> VEFNTDVLDAADKKNIDFTRFSEAGYVLPGQYLLDVIVNGQSISPASLQISFVEPQSSGDKAEKKLPQACLTSDMVRLMGLTAESLDKVVYWHDGQCADFHGLPGVDIRPDTGAGVLRINMPQARLEYSDATWLPPSRWDDGIPGLMLDYNLNGTVSRNYQGGDSHQFSYNGTVGGNLGPWRLRADYQGSQEQSRYNGEKTTNRNFTWSRFYLFRAIPRWRANLTLGENNINSDIFRSWSYTGASLESDDRMLPPRLRGYAPQITGIAETNARVVVSQQGRVLYDSMVPAGPFSIQDLDSSVRGRLDVEVIEQNGRKK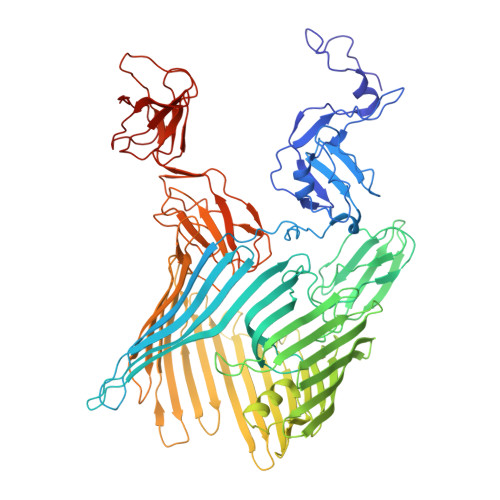TFQVDTASVPYLTRPGQVRYKLVSGRSRGYGHETEGPVFATGEASWGLSNQWSLYGGAVLAGDYNALAAGAGWDLGVPGTLSADITQSVARIEGERTFQGKSWRLSYSKRFDNADADITFAGYRFSERNYMTMEQYLNARYRNDYSSREKEMYTVTLNKNVADWNTSFNLQYSRQTYWDIRKTDYYTVSVNRYFNVFGLQGVAVGLSASRSKYLGRDNDSAYLRISVPLGTGTASYSGSMSNDRYVNMAGYTDTFNDGLDSYSLNAGLNSGGGLTSQRQINAYYSHRSPLANLSANIASLQKGYTSFGVSASGGATITGKDAALHAGGMSGGTRLLVDTDGVGGVPVDGGQVVTNRWGTGVVTDISSYYRNTTSVDLKRLPDDVEATRSVVESALTEGAIGYRKFSVLKGKRLFAILRLADGSQPPFGASVTSEKGRELGMVADEGLAWLSGVTPGETLSVNWDGKIQCQVNVPETAISDQQLLLPCTPQK(5S)-7-(2-fluoropyridin-3-yl)-3-[(3-methyloxetan-3-yl)ethynyl]spiro[chromeno[2,3-b]pyridine-5,4'-[1,3]oxazol]-2'-amine 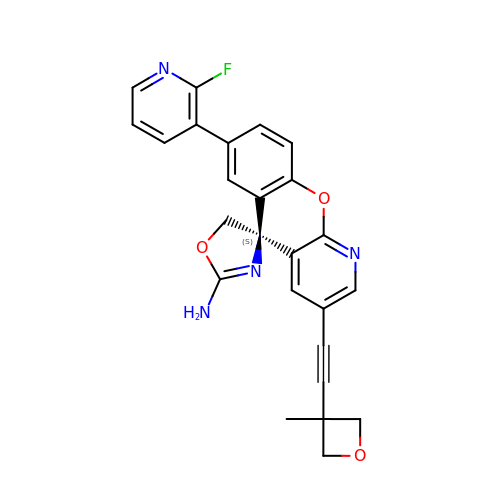| C25 H19 F N4 O3 | GKKFBOARESVMBW-VWLOTQADSA-N> MEIDPKDLTFLKELGTGQFGVVKYGKWRGQYDVAIRMIREGSMSEDEFIEEAKVMMNLSHEKLVQLYGVCTKQRPIFIITEYMANGCLLNYLREMRHRFQTQQLLEMCKDVCEAMEYLESKQFLHRDLAARNCLVNDQGVVKVSDFGMTRYVLDDEYTSSTGSKFPVKWASPEVLMYSKFSSKSDIWAFGVLMWEIYSLGKMPYERFTNSETAEHIAQGLRLPRPHLASERVYTIMYSCWHEKADERPSFKILLSNILDVMDEESHHHHHH

Bruton’s tyrosine kinase (BTK), is a non-receptor tyrosine kinase that is one of the five TEC family kinases expressed primarily in hematopoietic cells. BTK propagates signaling from the B-cell receptor, including B cells at very early stages of differentiation, as well as the Fc receptor, Toll-like receptors and chemokine receptors. In addition to its causative role in XLA, BTK is an essential signaling molecule for proliferation of leukemia and lymphoma cells in B cell malignancies. To facilitate crystal packing, we expressed the kinase domain of murine BTK (residues 396–659) with a kinase-inactive mutation, K430R, and substituted six residues in the activation loop with the corresponding residues from ITK (hereafter referred to as BTK KD), which we have previously shown stabilizes the activation loop in solution and has been employed in prior crystallization efforts.

Comparison of the BTK KD/acalabrutinib complex structure with the tirabrutinib bound BK KD shows large differences in the conformation of the activation loop. This is accompanied by extensive contacts between the side chain of Phe413 on the glycine rich loop and the activation loop that are not present in the acalabrutinib complex structure or any of the other inhibitor bound structures. To test the degree to which this unusual activation loop conformation might be related to tirabrutinib binding, we solved the structure of BTK KD/tirabrutinib complex structure via co-crystallization of BTK and tirabrutinib. The x-ray data was collected from the crystals in the PEG 8000 condition and the BTK KD/tirabrutinib complex structure was determined to 2.6Å. Tirabrutinib binding is identical in the two structures but the activation loop adopts very different conformations in the two structures. The activation loop conformation in our co-crystallized BTK KD/tirabrutinib complex is nearly identical to structures of the BTK kinase domain bound to ibrutinib, zanubrutinib and acalabrutinib. The RMSD for the activation loop residues 539–567 in our BTK KD/tirabrutinib structure the BTK KD complex with ibrutinib is 0.43 Å, with zanubrutinib is 0.58 Å, and with acalabrutinib is 0.46 Å. Thus, we interpret differences in the tirabrutinib complex we report here and that solved previously to suggest that the drug bound kinase domain undergoes dynamic fluctuations. Indeed, the activation loop conformation in the previous BTK KD/tirabrutinib structure is characterized by elevated B-factors compared to the rest of the structure and some side chain densities are not visible. Acalabrutinib and tirabrutinib both contain the butynamide ‘warhead’ instead of the acrylamide group found in ibrutinib, zanubrutinib and orelabrutinib.>[2x]MGSDKIHHHHHHMPKIWTERIFDDPEIYVLRIDDDRIRYFEAVWEIPEGISYNAYLVKLNGANVLIDGWKGNYAKEFIDALSKIVDPKEITHIIVNHTEPDASGSLPATLKTIGHDVEIIASNFGKRLLEGFY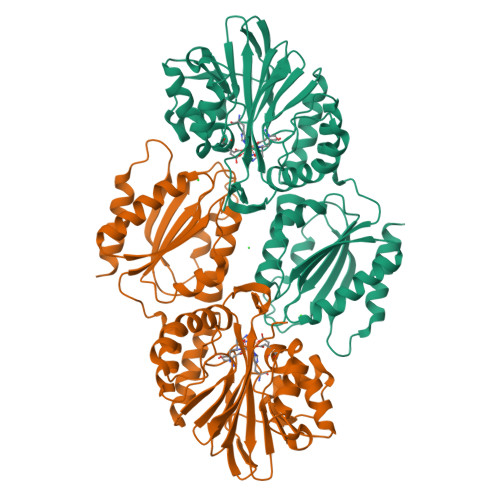GIKDVTVVKDGEEREIGGKKFKFVMTPWLHWPDTMVTYLDGILFSCDVGGGYLLPEILDDSNESVVERYLPHVTKYIVTVIGHYKNYILEGAEKLSSLKIKALLPGHGLIWKKDPQRLLNHYVSVAKGDPKKGKVTVIYDSMYGFVENVMKKAIDSLKEKGFTPVVYKFSDEERPAISEILKDIPDSEALIFGVSTYEAEIHPLMRFTLLEIIDKANYEKPVLVFGVHGWAPSAERTAGELLKETKFRILSFTEIKGSNMDERKIEEAISLLKKELE> MDTSNLMEQILSSDNLNRAYLQVVRNKGAEGVDGMKYTELKEHLAKNGETIKGQLRTRKYKPQPARRVEIPKPDGGVRNLGVPTVTDRFIQQAIAQVLTPIYEEQFHDHSYGFRPNRCAQQAILTALNIMNDGNDWIVDIDLEKFFDTVNHDKLMTLIGRTIKDGDVISIVRKYLVSGIMIDDEYEDSIVGTPQGGNLSPLLANIMLNELDKEMEKRGLNFVRYADDCIIMVGSEMSANRVMRNISRFIEEKLGLKVNMTKSKVDRPSGLKYLGFGFYFDPRAHQFKAKPHAKSVAKFKKRMKELTCRSWGVSNSYKVEKLNQLIRGWINYFKIGSMKTLCKELDSRIRYRLRMCIWKQWKTPQNQEKNLVKLGIDRNTARRVAYTGKRIAYVCNKGAVNVAISNKRLASFGLISMLDYYIEKCVTC

pmcGroup II introns are self-splicing retroelements that have played a key role in shaping eukaryotic genomes as the ancestors of spliceosomal introns and non-LTR retroelements. Group II introns encode a specialized reverse transcriptase (maturase or intron-encoded protein (IEP)), that binds its parent intron and facilitates self-splicing, releasing a well-folded lariat ribonucleoprotein (RNP) complex. The liberated RNP functions as a retrotransposon, targeting DNA that contains spliced exon junction sequences and inserting via a two-step transesterification reaction known as reverse splicing. Unlike their larger IIA and IIB counterparts, group IIC introns are almost completely dependent on their IEPs to facilitate intron excision through lariat formation, thereby forming the functional RNP that serves as the minimal element for retrotransposition.

We were surprised to observe that the apo-RNP has an architecture that is almost identical to that of the complex bound to DNA, and that substrate binding induces only minor changes in the structure. Most remarkably, the RNP active site remains completely intact. The maturase does not change its orientation in the absence of DNA, remaining coordinated at two anchor points along the D4a arm, with the thumb and DBD inserted into the active site to participate in catalysis. In this configuration, the binding interface for the target DNA is maintained, enabling the RNP to readily recognize an incoming DNA target and rapidly engage in retrotransposition. In previous ligand-free intron structures, EBS nucleotides were found to be disordered or rearranged. Here, we observe that the positions of the EBS nucleotides are unchanged, likely due to the presence of the maturase. These findings reinforce the mechanistic role of the protein as a stabilizing catalytic component. Further evidence of a pre-formed catalytic core includes the persistence of the heteronuclear metal ion cluster, which remains organized around the lariat, although M2 is not visible in this case. The apo-retroelement is completely poised to react and does not require any reorganization of structure upon target DNA binding. The arrangement of the active site, from substrate recognition nucleotides to the heteronuclear metal ion cluster to the DNA binding interface, is preserved despite the absence of DNA substrate.> GSEAAGGEQRELLIQRLRAAVHYTTGALAQDVAEDKGVLFSKQTVAAISEITFRQAEN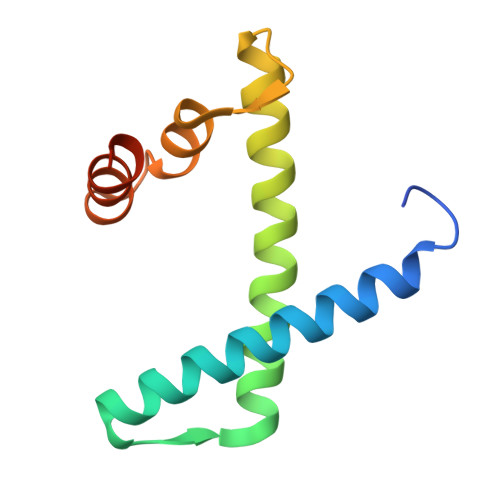FARDLEMFARHAKRSTITSEDVKLLARRSNSLLKYITQKSDELASSNME(4R)-4-{3-[hydroxy(methyl)amino]-3-oxopropyl}-L-glutamic acid | C9 H16 N2 O6 | 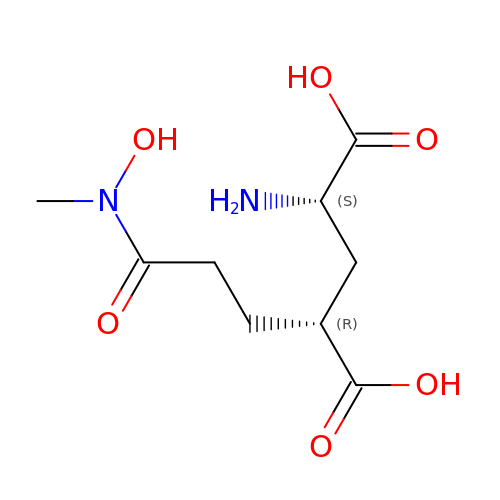YWTXUGAXXGHUOR-RITPCOANSA-N> SNNAVTHVSANSIRQHILFNNFETLHKDIQSKIDLVNTFTPQTKNLIFRNLLIVITNSYHLQNLLDALEQLEPMYVTDAYSEAILNEIGLCDKGIPNLSSIHFMIYLVSGLTKLTTKQSKILMEIVTDAK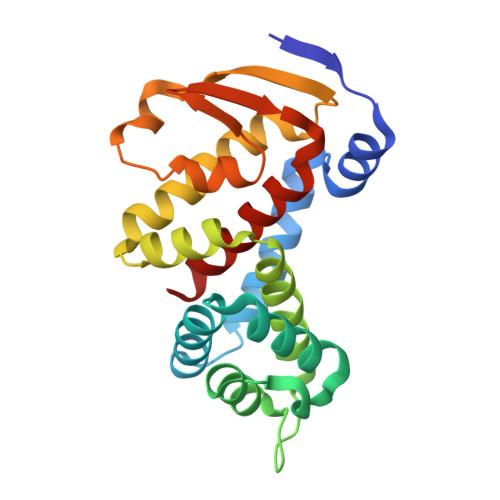IFCHHVNVLEYIIKKNVEKLETVTSTLLEKYTKLPLEVTLFKESGLKIQGNTYIWDPEHKKSICNLYTVIKIMSYIM> AEEKAKAVPLIHQEGNRLYREGHVKEAAAKYYDAIACLKNLQMKEQPGSPEWIQLDQQIT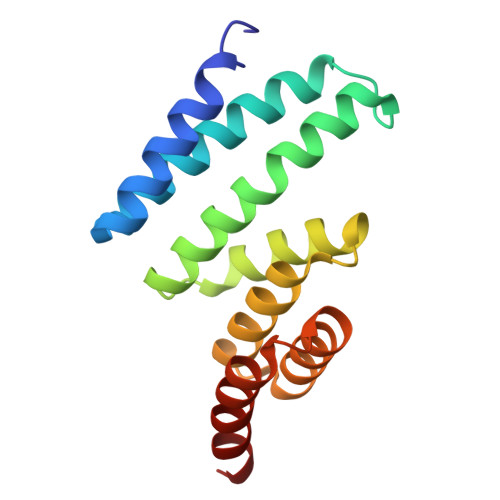PLLLNYCQCKLVVEEYYEVLDHCSSILNKYDDNVKAYFKRGKAHAAVWNAQEAQADFAKVLELDPALAPVVSRELQALEARIRQ> ASVQLQNVTKAWGE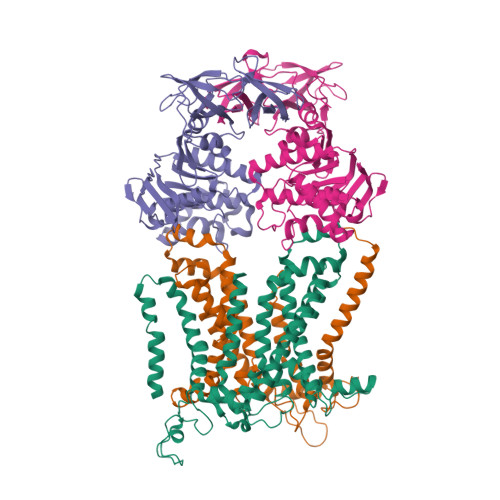VVVSKDINLDIHEGEFVVFVGPSGCGKSTLLRMIAGLETITSGDLFIGEKRMNDTPPAERGVGMVFQSYALYPHLSVAENMSFGLKLAGAKKEVINQRVNQVAEVLQLAHLLDRKPKALSGGQRQRVAIGRTLVAEPSVFLLDEPLSNLDAALRVQMRIEISRLHKRLGRTMIYVTHDQVEAMTLADKIVVLDAGRVAQVGKPLELYHYPADRFVAGFIGSPKMNFLPVKVTATAIDQVQVELPMPNRQQVWLPVESRDVQVGANMSLGIRPEHLLPSDIADVILEGEVQVVEQLGNETQIHIQIPSIRQNLVYRQNDVVLVEEGATFAIGLPPERCHLFREDGTACRRLHKEPGVA;> ASVQLQNVTKAWGEVVVSKDINLDIHEGEFVVFVGPSGCGKSTLLRMIAGLETITSGDLFIGEKRMNDTPPAERGVGMVFQSYALYPHLSVAENMSFGLKLAGAKKEVINQRVNQVAEVLQLAHLLDRKPKALSGGQRQRVAIGRTLVAEPSVFLLDEPLSNLDAALRVQMRIEISRLHKRLGRTMIYVTHDQVEAMTLADKIVVLDAGRVAQVGKPLELYHYPADRFVAGFIGSPKMNFLPVKVTATAIDQVQVELPMPNRQQVWLPVESRDVQVGANMSLGIRPEHLLPSDIADVILEGEVQVVEQLGNETQIHIQIPSIRQNLVYRQNDVVLVEEGATFAIGLPPERCHLFREDGTACRRLHKEPGVAHH;> MDVIKKKHWWQSDALKWSVLGLLGLLVGYLVVLMYAQGEYLFAITTLILSSAGLYIFANRKAYAWRYVYPGMAGMGLFVLFPLVCTIAIAFTNYSSTNQLTFERAQEVLLDRSWQAGKTYNFGLYPAGDEWQLALSDGETGKNYLSDAFKFGGEQKLQLKETTAQPEGERANLRVITQNRQALSDITAILPDGNKVMMSSLRQFSGTQPLYTLDGDGTLTNNQSGVKYRPNNQIGFYQSITADGNWGDEKLSPGYTVTTGWKNFTRVFTDEGIQKPFLAIFVWTVVFSLITVFLTVAVGMVLACLVQWEALRGKAVYRVLLILPYAVPSFISILIFKGLFNQSFGEINMMLSALFGVKPAWFSDPTTARTMLIIVNTWLGYPYMMILCMGLLKAIPDDLYEASAMDGAGPFQNFFKITLPLLIKPLTPLMIASFAFNFNNFVLIQLLTNGGPDRLGTTTPAGYTDLLVNYTYRIAFEGGGGQDFGLAAAIATLIFLLVGALAIVNLKATRMKFD;> AMVQPKSQKARLFITHLLLLLFIAAIMFPLLMVVAISLRQGNFATGSLWPEQISWDHWKLALGFSVEQADGRIWPPPFPVLLWLWNSVKVAGISAIGIVALSTTCAYAFARMRFPGKATLLKGMLIFQMFPAVLSLVALYALFDRLGEYIPFIGLNTHGGVIFAYLGGIALHVWTIKGYFETIDSSLEEAAALDGATPWQAFRLVLLPLSVPILAVVFILSFIAAITEVPVASLLLRDVNSYTLAVGMQQYLNPQNYLWGDFAAAAVMSALPITIVFLLAQRWLVN6-ethyl-5-[3-({3-[4-(trifluoromethyl)piperidin-1-yl]pyridin-2-yl}oxy)propoxy]pyrimidine-2,4-diamine 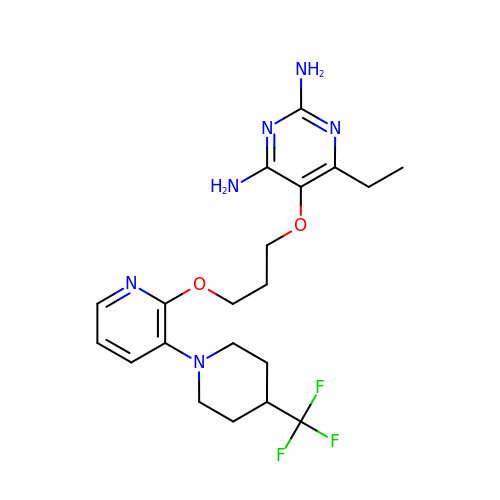| C20 H27 F3 N6 O2 | KHPDUBAKUFVHPS-UHFFFAOYSA-N9-[(4-chlorophenyl)methyl]-6-methoxy-1-methyl-4,9-dihydro-3H-beta-carboline | C20 H19 Cl N2 O | 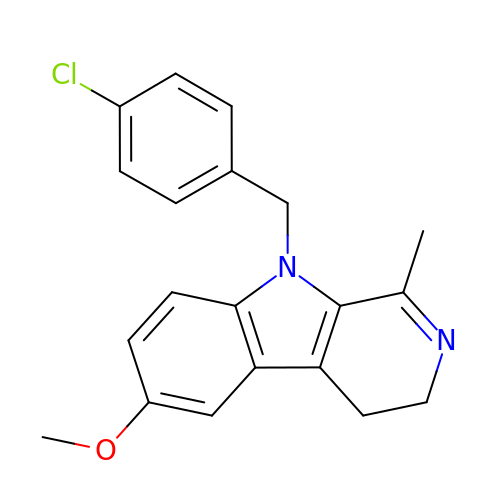SRMUEFRMPPZYOH-UHFFFAOYSA-N>[2x]GPGSMADPSLNNPVVIQATRLDASILPRNVFSKSYLLYVIAQGTDV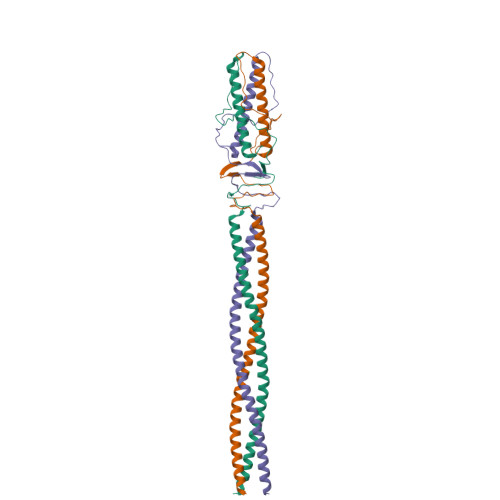GAIAGKANEAGQGAYDAQVKNDEQDVELADHEARIKQLRIDVDDHESRITANTKAITALNVRVTTAEGEIASLQTNVSALDGRVTTAENNISALQADYVSKTATTSQSLASPLNVTTSYSVGGKKVLGARQTGWTAATGTANKGVFDADLTFAVSDTYTQSEIQAIANALITERRRTKAMEDALRAHGLID> MKGKTAAGGGAICAIAVMITIVMGNGNVRTNQA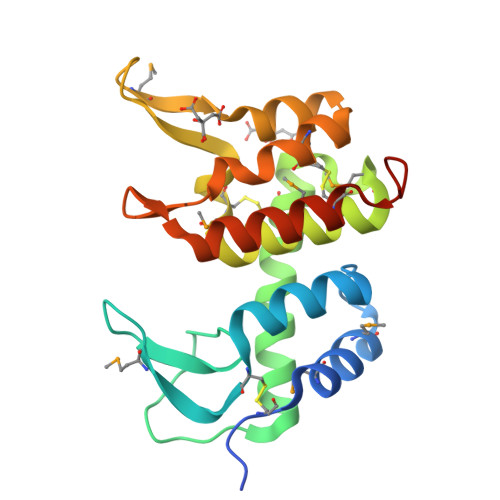GLELIGNAEGCRRDPYMCPAGVWTDGIGNTHGVTPGVRKTDQQIAADWEKNILIAERCINQHFRGKDMPDNAFSAMTSAAFNMGCNSLRTYYSKARGMRVETSIHKWAQKGEWVNMCNHLPDFVNSNGVPLRGLKIRREKERQLCLTGLVNEHHHHHH> TVPDRDNDGIPDSLEVEGYTVDVKNKRTFLS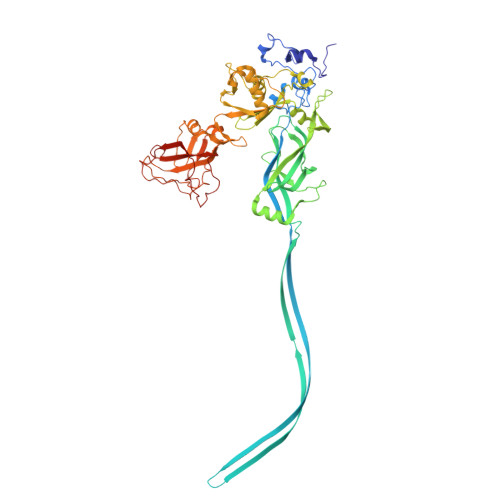PWISNIHEKKGLTKYKSSPEKWSTASDPYSDFEKVTGRIDKNVSPEARHPLVAAYPIVHVDMENIILSKNEDQSTQNTDSQTRTISKNTSTSRTHTSEVHGNAEVHASFFDIGGSVSAGFSNSNSSTVAIDHSLSLAGERTWAETMGLNTADTARLNANIRYVNTGTAPIYNVLPTTSLVLGKNQTLATIKAKENQLSQILAPNNYYPSKNLAPIALNAQDDFSSTPITMNYNQFLELEKTKQLRLDTDQVYGNIATYNFENGRVRVDTGSNWSEVLPQIQETTARIIFNGKDLNLVERRIAAVNPSDPLETTKPDMTLKEALKIAFGFNEPNGNLQYQGKDITEFDFNFDQQTSQNIKNQLAELNATNIYTVLDKIKLNAKMNILIRDKRFHYDRNNIAVGADESVVKEAHREVINSSTEGLLLNIDKDIRKILSGYIVEIEDTEGLKEVINDRYDMLNISSLRQDGKTFIDFKKYNDKLPLYISNPNYKVNVYAVTKENTIINPSENGDTSTNGIKKILIFSKKGYEIG> SNAMSDSLELSLDGVERRSLADFTEQAYLNYSMYVIMDRALPHIGDGLKPVQRRIVYAMSELGLDADAKHKKSARTVGDVLGKFHPHGDSACYEAMVLMAQPFSYRYTLVDGQGNWGAPDDPKSFAAMRYTEARLSRYAEVLLSEVGQGTVDWVPNFDGTLQEPAVLPARLPNILLNGTTGIAVGMATDVPPHNLREVASACVRLLDEPKATIEQLCEHIQGPDYPTEAEIVTPRAEILKMYESGRGSIRMRAVYRVEDGDIVVTALPHQVSGAKVLEQIAAQM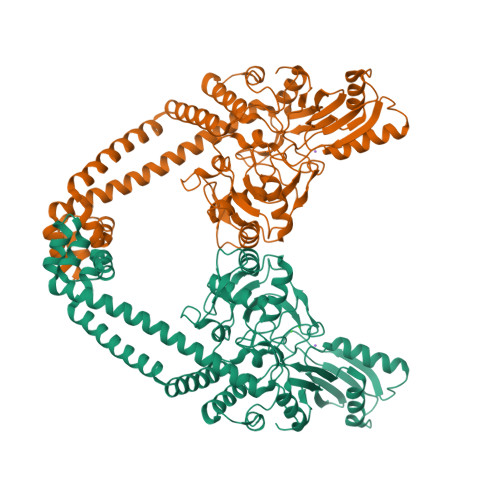QAKKLPMVADLRDESDHENPCRIVIIPRSNRVDVDELMQHLFATTDLESTYRVNVNIIGLDGRPQLKNLRTLLVEWLEFRTNTVRRRLQHRLDKVEKRLHLLDGLLTAFLNLDEVIHIIRTEEYPKQALIERFELTEIQADYILETRLRQLARLEEMKIRGEQDELLKEQAKLQALLGSEAKLRKLVRSELIKDAETYGDDRRSPIVARAEA The kinase-like nidovirus RdRp-associated nucleotidyl transferase (NiRAN) domain of nsp12 in SARS-CoV-2 catalyzes the formation of the 5′ RNA cap structure. To generate the RNA cap, the SARS-CoV-2 nsp12 nidovirus RdRp-associated nucleotidyl transferase (NiRAN) domain conjugates nascently transcribed RNA to nsp9 (RNAylation) and subsequently transfers the RNA to GDP, forming the core 5′ RNA cap structure GpppA-RNA. Although the NiRAN domain adopts a protein kinase fold, it acts as a GDP-polyribonucleotidyltransferase that catalyzes an essential step in the viral life cycle. Viral replication is abolished when mutations are introduced into key residues in the NiRAN domain or nsp9 that participate in the formation of the cap.

We identified NiRAN covalent inhibitor 2 (NCI-2), a compound with a reactive chloromethyl group that covalently binds to an active site cysteine (Cys53) in the NiRAN domain, inhibiting its activity. We determined a cryo-EM structure of the SARS-CoV-2 replication-transcription complex (RTC) bound to NCI-2. The Coulomb potential map clearly shows the density for the ligand and the covalent bond with Cys53. NCI-2 occupies the active site space responsible for interactions with nucleotide substrates and sterically prevents the “base-in” mode of binding. While there are no significant clashes with the “base-up” nucleotide orientation, several residues typically involved in catalysis and/or nucleotide phosphate binding adopt different orientations (Lys50, Lys73, and Arg116). NCI-2 binding causes major rearrangements of the active site when compared to the apo structure. The catalytic Lys73 is displaced from the salt bridge with Glu83 and is replaced by Arg116 that normally interacts with the nucleotide phosphates. Lys50 moves toward the back of the active site and forms electrostatic interactions with NCI-2. Additional electrostatic interactions are formed through an ordered water molecule (H2O5) with the Arg33 guanidinium and a main chain carbonyl of Lys121. The heterocyclic ring of the inhibitor forms extensive interactions with a hydrophobic patch formed by Val71 and Leu119, while the methyl ester group forms hydrophobic interactions with Tyr217 and Thr123.

> MGSSHHHHHHENLYFQSADAQSFLNRVCGVSAARLTPCGTGTSTDVVYRAFDIYNDKVAGFAKFLKTNCCRFQEKDEDDNLIDSYFVVKRHTFSNYQHEETIYNLLKDCPAVAKHDFFKFRIDGDMVPHISRQRLTKYTMADLVYALRHFDEGNCDTLKEILVTYNCCDDDYFNKKDWYDFVENPDILRVYANLGERVRQALLKTVQFCDAMRNAGIVGVLTLDNQDLNGNWYDFGDFIQTTPGSGVPVVDSYYSLLMPILTLTRALTAESHVDTDLTKPYIKWDLLKYDFTEERLKLFDRYFKYWDQTYHPNCVNCLDDRCILHCANFNVLFSTVFPPTSFGPLVRKIFVDGVPFVVSTGYHFRELGVVHNQDVNLHSSRLSFKELLVYAADPAMHAASGNLLLDKRTTCFSVAALTNNVAFQTVKPGNFNKDFYDFAVSKGFFKEGSSVELKHFFFAQDGNAAISDYDYYRYNLPTMCDIRQLLFVVEVVDKYFDCYDGGCINANQVIVNNLDKSAGFPFNKWGKARLYYDSMSYEDQDALFAYTKRNVIPTITQMNLKYAISAKNRARTVAGVSICSTMTNRQFHQKLLKSIAATRGATVVIGTSKFYGGWHNMLKTVYSDVENPHLMGWDYPKCDRAMPNMLRIMASLVLARKHTTCCSLSHRFYRLANECAQVLSEMVMCGGSLYVKPGGTSSGDATTAYANSVFNICQAVTANVNALLSTDGNKIADKYVRNLQHRLYECLYRNRDVDTDFVNEFYAYLRKHFSMMILSDDAVVCFNSTYASQGLVASIKNFKSVLYYQNNVFMSEAKCWTETDLTKGPHEFCSQHTMLVKQGDDYVYLPYPDPSRILGAGCFVDDIVKTDGTLMIERFVSLAIDAYPLTKHPNQEYADVFHLYLQYIRKLHDELTGHMLDMYSVMLTNDNTSRYWEPEFYEAMYTPHTVLQ;>[2x]AIASEFSSLPSYAAFATAQEAYEQAVANGDSEVVLKKLKKSLNVAKSEFDRDAAMQRKLEKMADQAMTQMYKQARSEDKRAKVTSAMQTMLFTMLRKLDNDALNNIINNARDGCVPLNIIPLTTAAKLMVVIPDYNTYKNTCDGTTFTYASALWEIQQVVDADSKIVQLSEISMDNSPNLAWPLIVTALRANSAVKLQ;> SKMSDVKCTSVVLLSVLQQLRVESSSKLWAQCVQLHNDILLAKDTTEAFEKMVSLLSVLLSMQGAVDINKLCEEMLDNRATLQ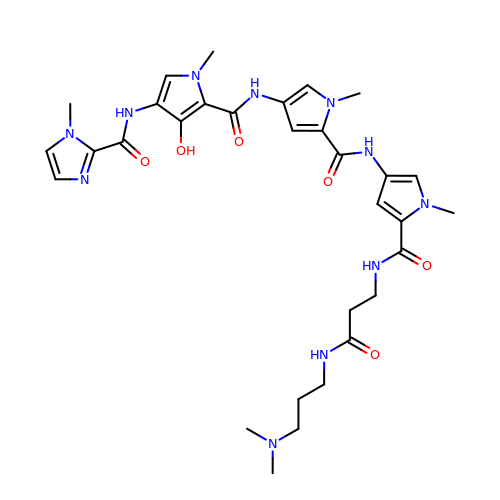~{N}-[5-[[5-[[5-[[3-[3-(dimethylamino)propylamino]-3-oxidanylidene-propyl]carbamoyl]-1-methyl-pyrrol-3-yl]carbamoyl]-1-methyl-pyrrol-3-yl]carbamoyl]-1-methyl-4-oxidanyl-pyrrol-3-yl]-1-methyl-imidazole-2-carboxamide | C31 H41 N11 O6 | LNQWOHIRWNQTSI-UHFFFAOYSA-N Encoded by the smallest of the eight viral genome segments, NS1 is a multifunctional RNA-binding protein, which is considered the main weapon of the virus to antagonize the innate immune response of the host and to ensure viral replication in a hostile anti-viral environment. While the effector domain is to some extent dispensable for the biological activities of NS1, the RBD plays an essential role in several activities that require the interaction of NS1 with viral and non-viral RNAs. This is best illustrated by the total loss of pathogenicity conferred by the alanine substitution of Arg38 and Lys41, the two main residues involved in binding of RNAs by NS1.

Based on this rationale, we designed a model double-stranded RNA made up by the annealing of two synthetic RNA molecules of the same sequence. This synthetic palindromic dsRNA, named AWFC01, harbors one GUAAC motif at each of its blunt ends and is perfectly symmetric thanks to a central uracil nucleotide that stabilizes the RNA duplex by forming a non-canonical U*U Hoogsteen base pair. To get insight into the sequence-specific recognition of the double stranded RNA by the RBD, we solved, at 1.75 Å resolution, the crystal structure of the complex associating the wild type H7N1-RBD to the AWFC01 duplex (wtH7N1-RDB/AWFC01). The overall structure of the RBD in the complex is identical to that found in the apo form, with minor side chain rearrangements at the binding interface of helix α2 residues R37, R38, and K41. The H7N1 RBD sits almost parallel to the dsRNA helix axis and overlays the minor and the major grooves of the duplex. The assembly buries 1173.8 Å2 of the RNA solvent-accessible area (17.1% of the total) and 1156.7 Å2 for the RBD (14.1% of the total). In the complex, the RNA keeps its A-form conformation but a curvature of about 20° is observed, stretching along base pairs 8 and 9 at one end of the duplex. All direct interactions between the H7N1 RBD and AWFC01 occur via phosphate/amino acid and sugar/amino acid H-bonds and none through base recognition. Surprisingly, this revealed that in the high affinity dsRNA (AWFC01), the RNA axis is bent in a non-symmetrical fashion, whereas in the two other complexes (aaH7N1-RBD/AWFC01 and wtH7N1-RBD/ZKO*), the RNA axis bend is distributed symmetrically from the centre of the duplex. For AWFC01, axis bending is at a maximum between the seventh and eighth basepair at one end of the duplex, right after the GUAAC sequence. Instead, we observed a pronounced asymmetry in the network of hydrogen bonds that links the dsRNA to the RBD, owing to the position of residue R38 in polypeptide chain A. This skewed network pulls the seventh nucleotide of the two RNA chains, thereby locally bending its axis and skewing the overall shape of the dsRNA.

>[2x]GSHMSDSNTITSFQVDCYLWHIRKLLSMRDMCDAPFDDRLRRDQKALKGRGSTLGLDLRVATMEGKKIVEDILKSET>MVMYSLPPEVLAALERVKARLNKVGEELEPISLRKAVRHYIETPGKLLRPLLLLT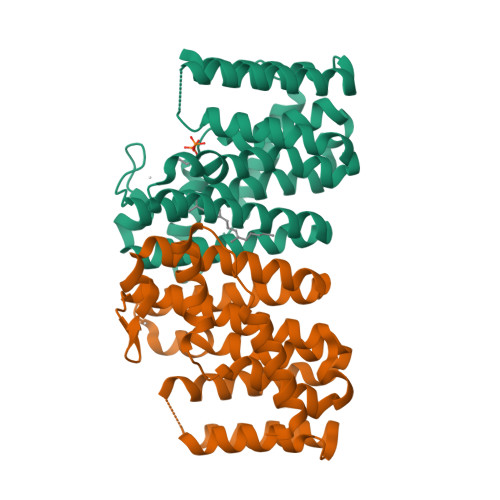FTYSIDRRSIMDPRILEAAAIVELLHVVSLLQDDVMDQHDQRRGIKTPRAMYGDGRAIVASDWLIAESIKMAVNLGADVVTYLADVAQRLSVGQALDLEGERDKAAEFKTAPLIEAALVMPLVILGRRELIETAKKLGTKLGILYQYSDDYSDENVERPETKSIANEIGRYLLKIKEHVGDAIAPFERLIKYLIGKALEGTLTVSRTIAENLYFQSHHHHHHWSHPQFEK[2x]> EVNTA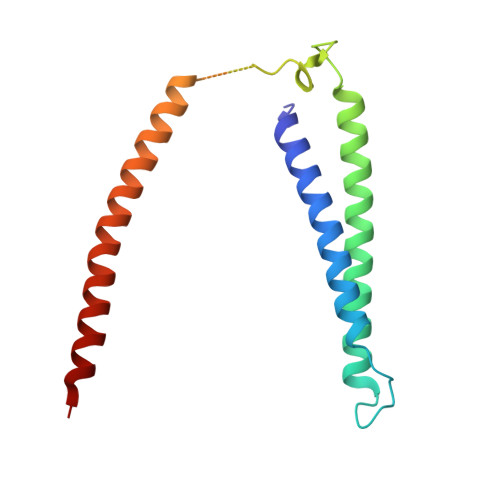TLCRIGQETVQDIVYRTMEIFQLLRNMQLPNGVTYHTGTYQDRLTKLQDHLRQLSILFRKLRLVYDKCNENCGGMDPIPVEQLIPYVDEDGSKNDDRAGPPRFASEERREIVEVNKKLKQKNQQLKQIMDQLRNLIWDINAMLAMRN N-FORMYLPIPERIDINE | C6 H11 N O | 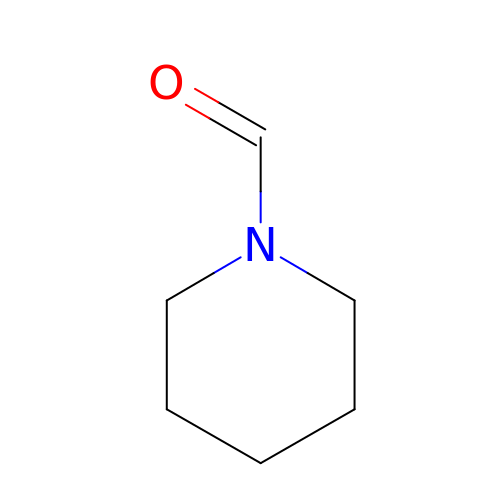FEWLNYSYJNLUOO-UHFFFAOYSA-N> MGHHHHHHHHHHSSGHIEGRHMFSKNAVKLHATPPSVAAPPTGAPEVAAERLEPRVEEKDGYWILKEQFRKGINPQEKVKIEKEPMKLFMENGIEELAKIPIEEIDQSKLTKDDIDVRLKWLGLFHRRKNQYGRFMMRLKLPNGVTTSAQTRYLASVIRKYGKEGCADITTRQNWQIRGVVLPDVPEILKGLAEVGLTSLQSGGDNVRNPVGNPLAGIDPEEIVDTRPYTNLLSQFITGNSRGNPAVSNLPRKWNPCVVGSHDLYEHPHINDLAYMPATKDGRFGFNLLVGGFFSAKRCDEAIP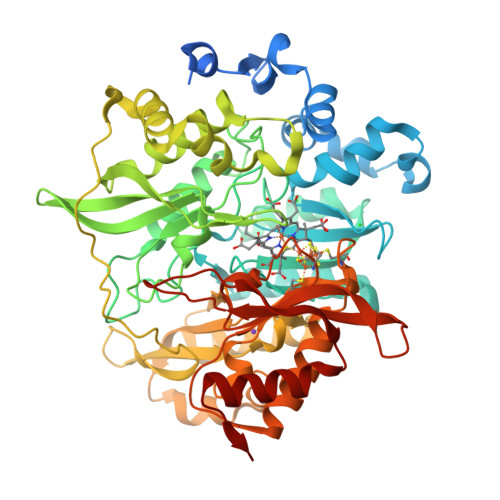LDAWVPADDVVPVCRAILEAFRDLGFRGNRQKCRMMWLIDELGVEGFRAEVEKRMPQQQLERASPEDLVQKQWERRDYLGVHPQKQEGYSFIGLHIPVGRVQADDMDELARLADEYGSGEIRLTVEQNIIIPNIETSKIEALLKEPVLSTFSPDPPILMKGLVACTGNQFCGQAIIETKARSLKITEEVQRQVSLTKPVRMHWTGCPNTCAQVQVADIGFMGCLTRDKNGKTVEGADVFLGGRIGSDSHLGEVYKKAVPCDDLVPLVVDLLVNNFGAVPR>SNAMIIADNIKQFHSIRNSLIKQQKIGFVPTMGALHNGHISLIKKAKSENDVVIVSIFVNPTQFNNPNDYQTYPNQLQQDIQILASLDVDVLFNPSEKDIYPDGNLLRIEPKLEIANILEGKSRPGHFSGMLTVV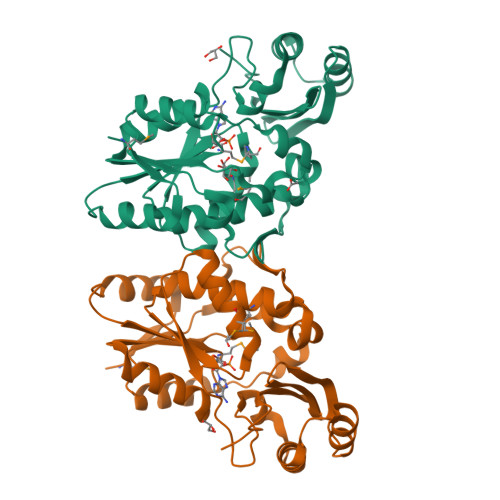LKLLQITKPNNLYLGEKDYQQVMLIKQLVKDFFINTKIIVCPTQRQPSGLPLSSRNKNLTSTDIEIANKIYEILRQDDFSNLEELTNKINSTGAKLQYIQKLNNRIFLAFYIGKVRLIDNFLKETGPSC[2x]>ASGNARIGKPAPDFKATAVVDGAFKEVKLSDYKGKYVVLFFYPLDFTFVCPTEIIAFSNRAEDFRKLGCEVLGVSVDSQFTHLAWINTPRKEGGLGPLNIPLLADVTRRLSEDYGVLKTDEGIAYRGLFIIDGK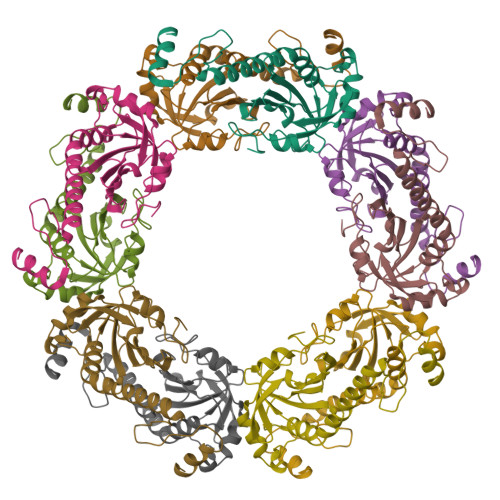GVLRQITVNDLPVGRSVDEALRLVQAFQYTDEHGEVSPAGWKPGSDTIKPNVDDSKEYFSKHN[10x]>MSTTQTPDLDAIVIGAGFGGIYMLHKLRNDLGLSVRVFEKGGGVGGTWYWNKYPGAKSDTEGFVYRYSFDKELLREYDWTTRYLDQPDVLAYLEHVVERYDLARDIQLNTEVTDAIFDEETELWRVTTAGGETLTARFLVTALGLLSRSNIPDIPGRDSFAGRLVHTNAWPEDLDITGKRVGVIGTGSTGTQFIVAAAKMAEQLTVFQRTPQYCVPSGNGPMDPDEVARIKQNFDSIWDQVRSSTVAFGFEESTVEAMSVSESERQRVFQQAWDKGNGFRFMFGTFCDIATNPEANAAAAAFIRSKIAEIVKDPETARKLTPTDLYAKRPLCNEGYYETYNRDNVSLVSLKETPIEEIVPQGVRTSDGVVHELDVLVFATGFDAVDGNYRAMNLRGRDGRHINEHWTEGPTSYLGVTKAGFPNMFMILG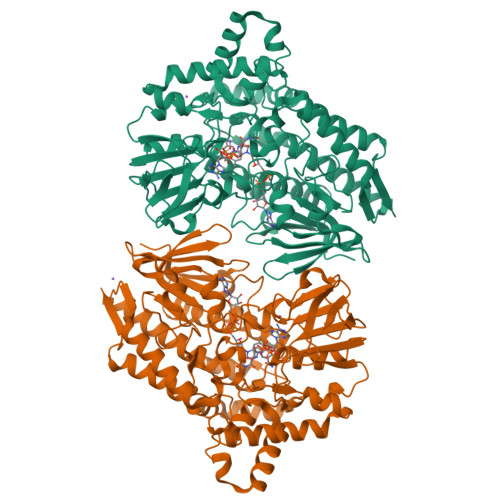PNGPFTNTPPSIEAQVEWISDLIDKATREGLTTVEPTADAEREWTETCAEIANMTLFPKADSWIFGANIPGKRHAVMFYLGGLGNYRRQLADVADGGYRGFQLRGERAQAVA[2x]> STLYEKLGGTTAVDLAVDKFYERVLQDDRIKHFFADVDMAKQRAHQKAFLTYAFGGTDKYDGRYMREAH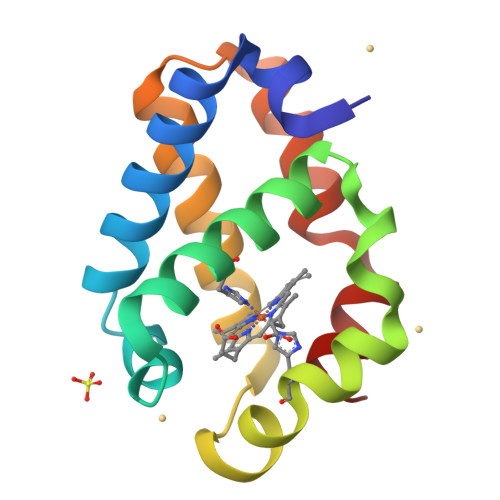KELVENHGLNGEHFDAVAEDLLATLKEMGVPEDLIAEVAAVAGAPAAKRDVLNQ> MSVEKIPGYTYG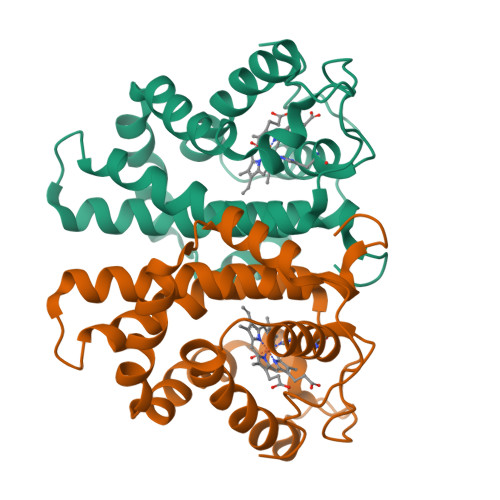ETENRAPFNLEDLKLLKEAVMFTAEDEEYIQKAGEVLEDQVEEILDTWWGFVGSHPHLLYYFTSPDGTPNEKYLAAVRKRFSRWILDTSNRSYDQAWLDYQYEIGLRHHRTKKNQTDNVESVPNIGYRYLVAFIYPITATMKPFLARKGHTPEEVEKMYQAWFKATTLQVALWSYPYVKYGDF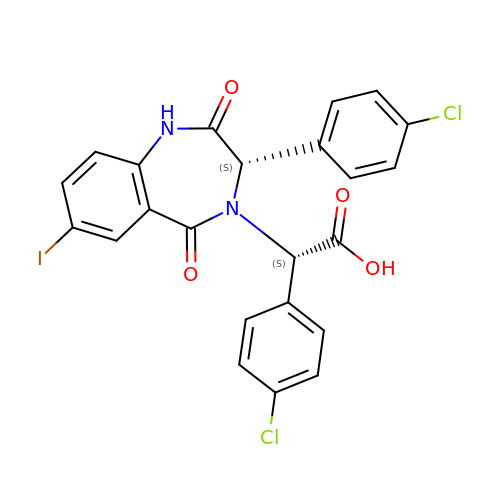(4-CHLOROPHENYL)[3-(4-CHLOROPHENYL)-7-IODO-2,5-DIOXO-1,2,3,5-TETRAHYDRO-4H-1,4-BENZODIAZEPIN-4-YL]ACETIC ACID | C23 H15 Cl2 I N2 O4 | HQEQUYKKMMKSSX-PMACEKPBSA-N> ANIVGGIEYSINNASLCSVGFSVTRGATKGFVTAGHCGTVNATARIGGAVVGTFAARVFPGNDRAWVSLTSAQTLLPRVANGSSFVTVRGSTEAAVGAAVCRSGRTTGYQCGTITAKNVTANYAEGAVRGLTQGNACMGRGDSGGSWITSAGQAQGVMSGGNVQSNGNNCGIPASQRSSLFERLQPILSQYG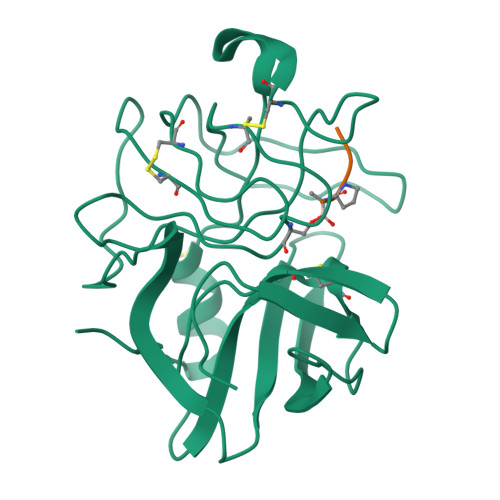LSLVTG;> XAAPA>[2x]PSVYDAAAQLTADVKKDLRDSWKVIGSDKKGNGVALMTTLFADNQETIGYFKRLG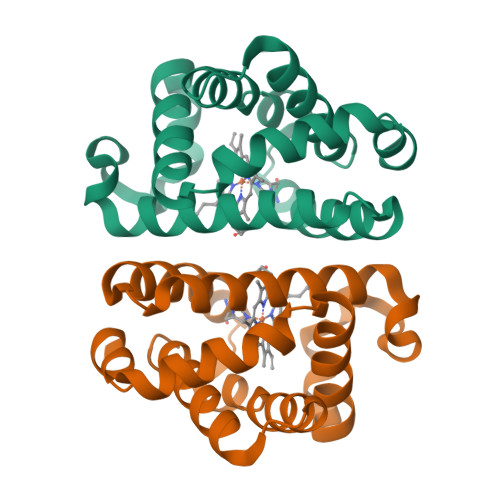DVSQGMANDKLRGHSITLMYALQNFIDQLDNPDDLVCVVEKYAVNHITRKISAAEFGKINGPIKKVLASKNFGDKYANAWAKLVAVVQAAL> DVSALAYVMLGLLLSLLNRLSLAAEAYKKAIELDPNDALAWLLLGSVLEKLKRLDEAAEAYKKAIELKPNDASAWKELGKV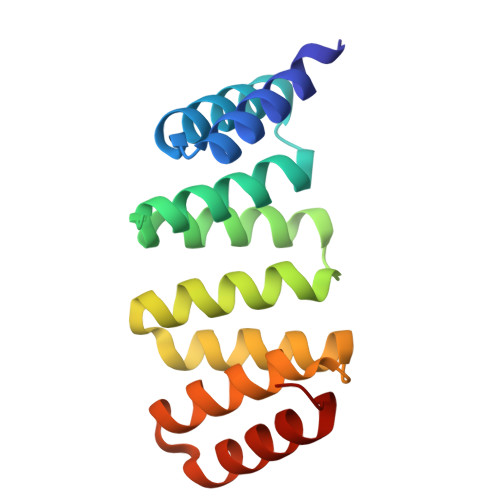LEKLGRLDEAAEAYLIAIMLDPEDAEAAKELGKVLEKLGELEMAEEAYKLAIKLDPND> GSEPAMEPETLEARINRATNPLNKELDWASINGFCEQLNEDFEGPP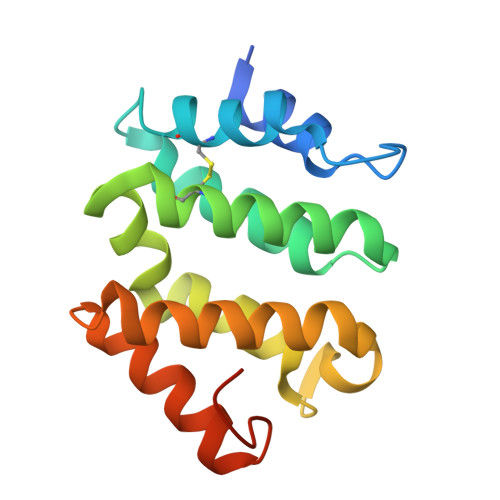LATRLLAHKIQSPQEWEAIQALTVLETCMKSCGKRFHDEVGKFRFLNELIKVVSPKYLGSRTSEKVKNKILELLYSWTVGLPEEVKIAEAYQMLKKQGIVKSDPKLPDDTTF> MAMFEQMRANVGKLLKGIDRYNPENLATLERYVETQAKENAYDLEANLAVLKLYQFNPAFFQTTVTAQILLKALTNLPHTD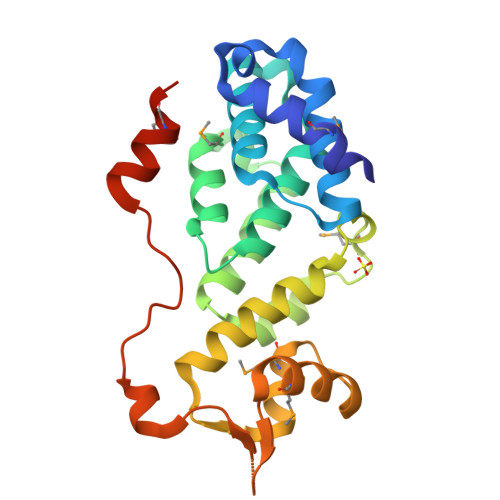FTLCKCMIDQAHQEERPIRQILYLGDLLETCHFQAFWQALDENMDLLEGITGFEDSVRKFICHVVGITYQHIDRWLLAEMLGDLSDSQLKVWMSKYGWSADESGQIFICSQEESIKPKNIVEKIDFDSVSSIMASSQLEHHHHHH> MTRETERFPAREFQRDLLDWFARERRDLPWRKDRDPYKVWVSEVMLQQTRVETVIPYFEQFIDRFPTLEALADADEDEVLKAWEGLGYYSRVRNLHAAVKEVKTRYGGKVPDDPDEFSRLKGVGPYTVGAVLSLAYGVPEPAVDGSVMRVLSRLFLVTDDIAKPSTRKRFEQIVREIMAYENPGAFNEALIELGALVCTPRRPSCLLCPVQAYCQAFAEGVAEE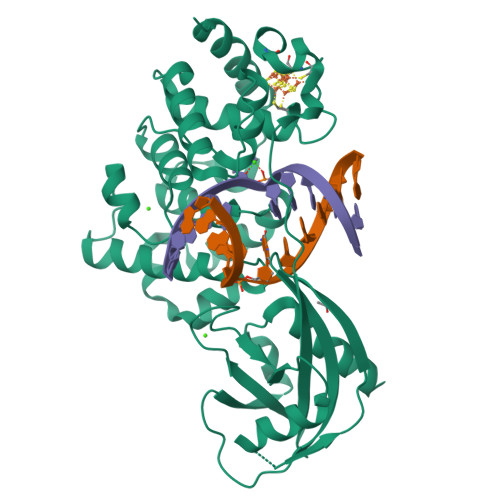LPVKMKKTAVKQVPLAVAVLADDEGRVLIRKRDSTGLLANLWEFPSCETDGADGKEKLEQMVGEQYGLQVELTEPIVSFEHAFSHLVWQLTVFPGRLVHGGPVEEPYRLAPEDELKAYAFPVSHQRVWREYKEWASGVRRP We report the biochemical and structural characterisation of a beta-carbonic anhydrase (β-CA) from Trichomonas vaginalis, a unicellular parasite responsible for one of the world’s leading sexually transmitted infections, trichomoniasis. CAs catalyse reversible CO2 hydration to bicarbonate and proton. CAs are divided into eight genetic families: α, β, γ, δ, ζ, η, θ, and ι14–17, which can vary in terms of amino acid sequence, oligomeric state, kinetics, and inhibition and activation profiles. α-CAs are the only isoforms present in humans, whereas many pathogens have been discovered with only β- and/or γ-CA genes in their genome. Here, we illustrate a full biochemical characterisation of TvaCA1, together with its crystallographic structure, thus providing the first detailed characterisation of a protozoan β–CA.

The crystals belonged to the space group P212121, with two molecules per asymmetric unit, and diffracted to a 2.48 Å resolution. In agreement with light-scattering experiment results, the two molecules in the asymmetric unit form a tightly associated dimer characterised by a buried surface area of approximately 4366 Å2 and many hydrogen bonds and van der Waals interactions at the interface between subunits. The dimer formation produces an extended β-sheet core consisting of ten β–strands, where the N-terminal helix of each monomer extends around the other monomer. There are two active sites per dimer, which are located in clefts at the dimeric interface. Each active site contains a zinc ion on the bottom, which is coordinated by three protein residues, Cys37, His96 and Cys99. In one of the two active sites, a water molecule is clearly visible in the fourth coordination position (Figure 4(B,C)), whereas in the other active site, this water molecule is not visible, probably due to the lower quality of the electron density maps in this region. Our crystallographic analysis clearly indicates that TvaCA1 belongs to the type I subclass. Indeed, even if the water molecule in the fourth coordination position is clearly visible only in one active site of the dimer, the aspartic acid residue, which is coordinated to the zinc ion in Type II β-CAs (Asp39 in the TvaCA1 sequence), is in both TvaCA1 active sites, very well defined in the electron density maps and far from the catalytic metal, leaving the active site in the open conformation. As observed for other β-CAs so far structurally characterised, the TvaCA1 active site is located in a narrow cavity spanning from the protein surface to the catalytic zinc ion. The comparison between the TvaCA1 catalytic cavity and that of human CAs showed significant differences in dimensions, being the latter much larger and more accessible.

>MSQLELITSANQAFLEANPELTKLNKAPQRHIAIVTCMDTRLVNFAEDAIGVKRGEATVIKAAGNGIWTTGLSDIVVSLLVSIYELGVQEIFIMGHECCGMTHASTDSLGAQMLKSGIKPEDIEKFKSDLSKWVDDFKDPIDNIKNSVRCVRENPLIPKNIPIHGLLIHPDTGKVTTIINGY[2x]> TRYWNAKAL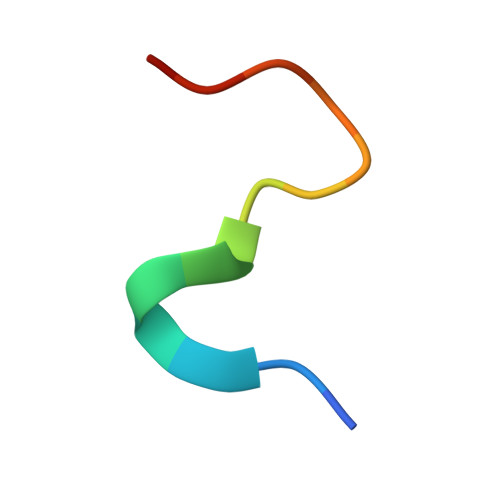PFAFGA4-nitrophenyl beta-D-galactopyranoside | C12 H15 N O8 | 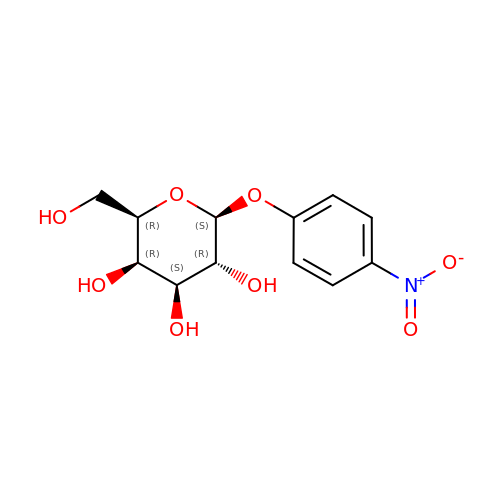IFBHRQDFSNCLOZ-YBXAARCKSA-N> GAMGSMWKRSEQMKIKSGKCNMAAAMETEQLGVEIFETADCEENIESQDRPKLEPFYVERYSWSQLKKLLADTRKYHGYMMAKAPHDFMFVKRNDPDGPHSDRIYYLAMSGENRENTLFYSEIPKTINRAAVLMLSWKPLLDLFQATLDYGMYSREEELLRERKRIGTVGIASYDYHQGSGTFLFQAGSGIYHVKDGGPQGFTQQPLRPNLVETSCPNIRMDPKLCPADPDWIAFIHSNDIWISNIVTREERRLTYVHNELANMEEDARSAGVATFVLQEEFDRYSGYWWCPKAETTPSGGKILRILYEENDESEVEIIHVTSPMLETRRADSFRYPKTGTANPKVTFKMSEIMIDAEGRIIDVIDKELIQPFEILFEGVEYIARAGWTP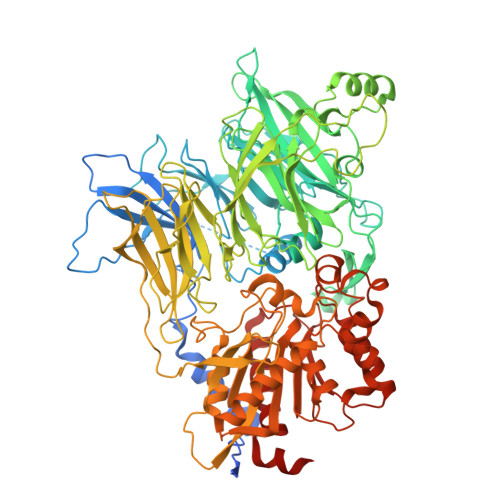EGKYAWSILLDRSQTRLQIVLISPELFIPVEDDVMERQRLIESVPDSVTPLIIYEETTDIWINIHDIFHVFPQSHEEEIEFIFASECKTGFRHLYKITSILKESKYKRSSGGLPAPSDFKCPIKEEIAITSGEWEVLGRHGSNIQVDEVRRLVYFEGTKDSPLEHHLYVVSYVNPGEVTRLTDRGYSHSCCISQHCDFFISKYSNQKNPHCVSLYKLSSPEDDPTCKTKEFWATILDSAGPLPDYTPPEIFSFESTTGFTLYGMLYKPHDLQPGKKYPTVLFIYGGPQVQLVNNRFKGVKYFRLNTLASLGYVVVVIDNRGSCHRGLKFEGAFKYKMGQIEIDDQVEGLQYLASRYDFIDLDRVGIHGWSYGGYLSLMALMQRSDIFRVAIAGAPVTLWIFYDTGYTERYMGHPDQNEQGYYLGSVAMQAEKFPSEPNRLLLLHGFLDENVHFAHTSILLSFLVRAGKPYDLQIYPQERHSIRVPESGEHYELHLLHYLQENLGSRIAALKVI Mitochondrial transcription factor B1 (TFB1M) is a dimethyltransferase that maintains mitochondrial homeostasis by catalyzing dimethylation of two adjacent adenines located in helix45 (h45) of 12S rRNA. This m62A modification is indispensable for the assembly and maturation of human mitochondrial ribosomes. TFB1M was originally thought to serve as a transcription factor along with TFB2M but has instead been shown to be a dimethyltransferase with the main role of m62A modification of the 3′ end of mitochondrial 12S rRNA. To clarify the mechanism of m62A modification, we determined the crystal structures of a ternary complex of human (hs) TFB1M (hsTFB1M–h45–SAM) and a binary complex (hsTFB1M–h45) both at 3.0 Å resolution.

Comparison of these two complexes revealed identical fold conformation of hsTFB1M and h45 appearing at an approximate 10° rotation only in the stem, possibly formed by base stacking. In the structures, the ‘GGAA’ tetraloop of 12S h45 flipped out to interact with hsTFB1M. The N-terminal domain (residues 28–236; residues 33–236 could be seen in the structure) formed a canonical Rossman-like methyltransferase fold with a central seven-stranded β-sheet flanked by three α-helices on each side. The C-terminal domain (residues 237–324) contained four α-helices (α7–α10) that likely formed a scaffold for other functional proteins. Electrostatic potential surface maps showed a positively-charged region located in the C-terminus of hsTFB1M, with interactions formed between Arg183, Arg256, and Arg257 and the phosphate backbone of h45. Electrostatic interactions between the phosphate backbones of h45 and positively-charged residues in hsTFB1M were critical for binding. Conversely, in the crystal structure, the four nucleotides in the ‘GGAA’ tetraloop all flipped out in order to interact with hsTFB1M, either for anchoring or modification.

> MQAAKQLSQNFLLDLRLTDKIVRKAGNLTNAYVYEVGPGPGGITRSILNADVAELLVVEKDTRFIPGLQMLSDAAPGKLRIVHGDVLTFKVEKAFSESLKRPWEDDPPNVHIIGNLPFSVSTPLIIKWLENISCRDGPFVYGRTQMTLTFQKEVAERLAANTGSKQRSRLSVMAQYLCNVRHIFTIPGQAFVPKPEVDVGVVHFTPLIQPKIEQPFKLVEKVVQNVFQFRRKYCHRGLRMLFPEAQRLESTGRLLELADIDPTLRPRQLSISHFKSLCDVYRKMCDEDPQLFAYNFREELKRRKSKNEEKEEDDAENYRL> ETLVRPKPLLLKLLKSVGAQKDTYTMKEVLFYLGQYIMTKRLYDEKQQHIVYCSNDLLGDLFGVPSFSVKEHRKIYTMIYRNL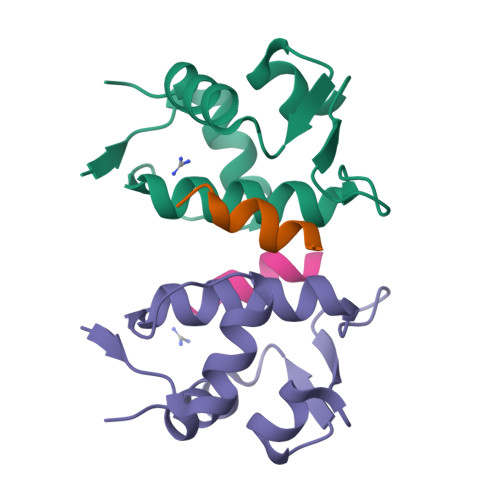VV;> TSFAEYWNLLSP>HPETLVTVKDIESRLGARVGYAVLDTASGKIWESYRADERFPMMSTFKVLACGALLSRVDAGQEQLDRRIRFRQSDLVTYSPVTEKHLDDGMTLAELCEAAITMSDNTAGNLVLETLGGPEGLTAFLRTLGDQVTRLDRWETALNEATPGDERDTTTPAAMAATLRKLLTGDALSPASRQQLIDWMEADKVAGPLLRSALPAGWFIADKSGAGGRGSRGIVAALGPPGKPPRIVVIYLTETEATMDERNAAIAEIGAALIKHW[2x]

The TEM-1 β-lactamase model system has been extensively used to study protein evolution. β-lactamases are a class of enzymes that are produced by bacteria in order to provide resistance to bactericidal β-lactam antibiotics through hydrolysis of their core β-lactam ring. We apply EVcouplings to computationally design variants of the model protein TEM-1 β-lactamase. To examine the structural effects of these mutations, we obtained X-ray crystal structures of designs 80.a, 80.b, and 70.a. Aligning these structures in 3D to a published WT TEM-1 structure (PDB: 1XPB34) revealed that all three have nearly identical Cα backbones to WT TEM-1 (0.26–0.61 Å RMSD over all Cα atoms).

We also searched for local structural changes by examining differences in all pairwise distances between residues, which showed small changes in a one looped region for all three structures (positions 255–257) and in a second loop of 70.a (positions 53–55). Both 80.a and 80.b have 55 amino acid substitutions relative to WT TEM-1, of which 80.a has 15 mutations in the core of the structure and 80.b has 19 in the core. The 80.a and 80.b designs also had a 4-fold increased MIC of aztreonam, as well as a 16-fold increased MIC of ceftazidime. The two designs that were optimized solely for predicted fitness (i.e., distance unconstrained) both conferred resistance to ampicillin, with the greedy optimized sequence (opt.a) having a MIC equal to WT TEM-1, and the parallel tempering optimized sequence (opt.b) had a large decrease in MIC (roughly 100X less). In summary, nearly all of the designs were able to confer resistance to ampicillin including a design with 84 mutations relative to its closest natural homolog (70.a) and two designs with over 50 mutations (80.a and 80.b). Most of the rest of the distance-constrained designs (98.a, 98.b, 95.a, 95.b, and 80.b), which all had more than an 11 °C increased melting temperature, also had increased activity on at least one of the four tested β-lactams. To investigate the structural basis for the increased Tm (80.a had a 24 °C increase relative to WT TEM-1, 80.b had a 18 °C increase, and 70.a had a 6.3 °C increase), we tallied the total number of hydrogen bonds and the number of atom pairs in contact (1.7–4 Å) in each structure. However, we did observe literature-reported globally stabilizing mutations such as M182T in every one of the designed sequences, which has been shown to confer a 7.5 °C increase in Tm as a single substitution. The 70.a, 80.a and 80.b designs also showed increased resistance to aztreonam (80.a and 80.b had a 4-fold increased MIC, and 70.a had a 32-fold increase MIC, see broth microdilution assay in Figs. 4, 5). There are five shared mutations near the active site that are in three designs (M69A, E104T, P167T, E168A, E240G) that may contribute to this increased resistance.> SITENTSWNKEFSAEAVNGVFVLCKSSSKSCATNDLARASKEYLPASTFKIPNAIIGLETGVIKNEHQVFKWPGKPRAMKQWERDLTLRGAIQVSAVPVFQQIAREVGEVRMQKYLKKFSYGNQNISGGI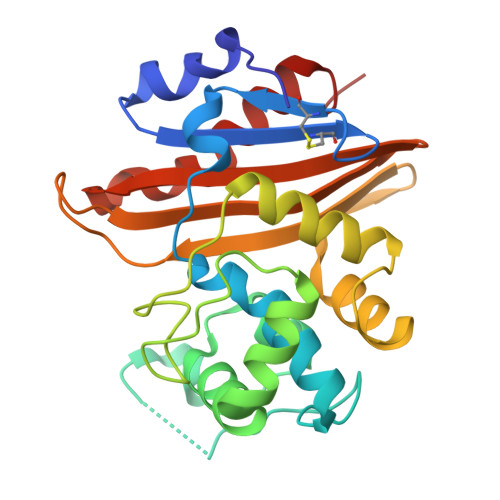DKFWLEGQLRISAVNQVEFLESLYLNKLSASKENQLIVKEALVTEAAPEYLVHSKTGFSGVGTESNPGVAWWVGWVEKETEVYFFAFNMDIDNESKLPLRKSIPTKIMESEGIIGG> GPGDQRFGDLVFRQLAPNVWQHTSYLDMPGFGAVASNGLIVRDGGRVLVVDTAWTDDQTAQILNWIKQEINLPVALAVVTHAHQDKMGGMDALHAAGIATYANALSNQLAPQEGLVAAQHSLTFAANGWVEPATAPNFGPLKVFYPGPGHTSDNITVGIDGTDIA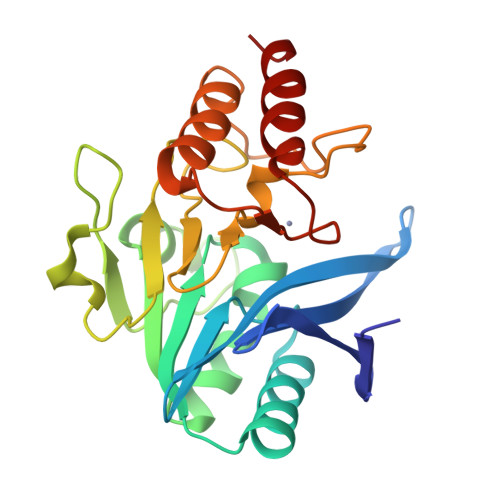FGGCLIKDSKAKSLGNLGDADTEHYAASARAFGAAFPKASMIVMSHSAPDSRAAITHTARMADKLR>KLCLVCSDEASGCHYGVLTCGSCKVFFKRAVEGQHNYLCAGRNDCIIDKIRRKNCPACRYRKCLQAGMNL[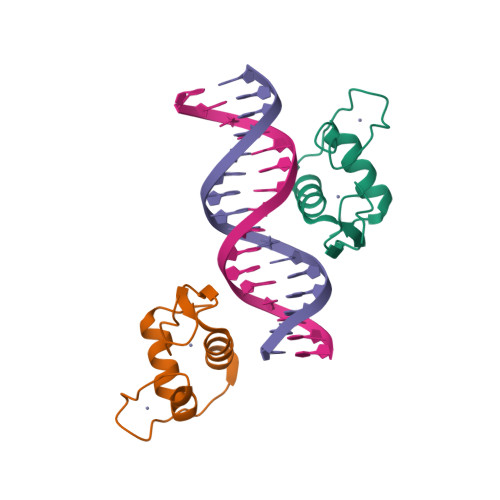2x]>[2x]NAKASKASLDFKRYVTDRRLAETLAQIYLGKPSRPPHLLLECNPGPGILTQALLEAGAKVVALESDKTFIPHLESLGKNLDGKLRVIHCDFFKLDPRSGGVIKPPAMSSRGLFKNLGIEAVPWTADIPLKVVGMFPSRGEKRALWKLAYDLYSCTSIYKFG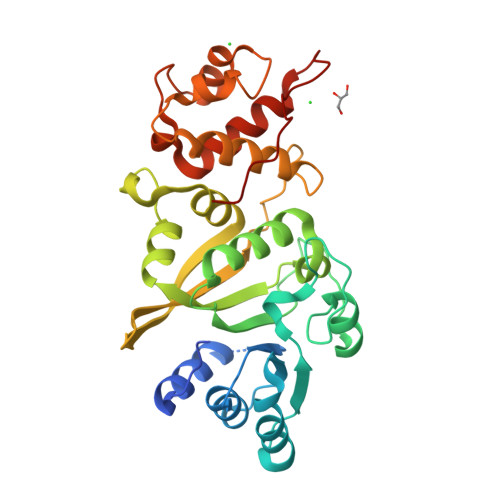RIEVNMFIGEKEFQKLMADPGNPDLYHVLSVIWQLACEIKVLHMEPGSSGKLYLIQMIPRQNLFTKNLTPMNYNIFFHLLKHCFGRRSATVIDHLRSLTPLDARDILMQIGKQEDEKVVNMHPQDFKTLFETIERSKDCAYKWLYDETLEDR> EXCQKWMWTCDSARACCEGLRC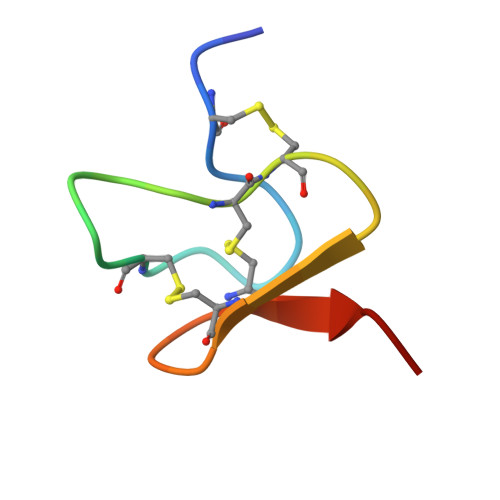KLWCRKEIX>GSASKSISDISFEVDRLAGQVSAFETVINKGGKVEEKSLVNLIEMLMNQLLRLDAIIADGDVKLMRKMQVQRVQKYVEA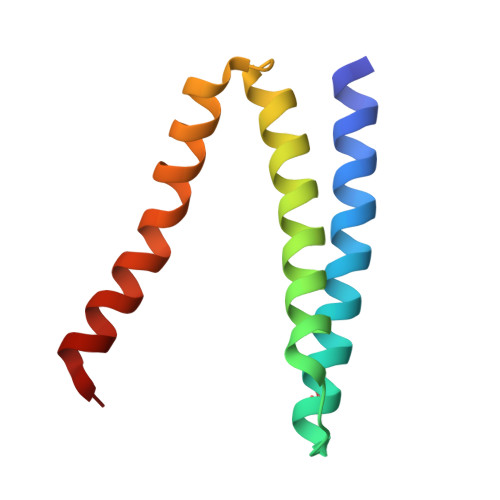LDLLKVKNS[2x]>[4x]MPRIIELRQQKTAIKNQMRDMLENAEKENRSLNDAEGAKFDELRAKAESLDKDISRLEAIADEERSKPGKSSQTTDPAELRNYILTGETRALSTGVPADGGYTVIPELNTEIMRMLTDESTMRRICTVKKISSNEFKQLVSAGGATVNHGEEGKTREQTSTPQINEVSIKLYPVYAYPRTTQE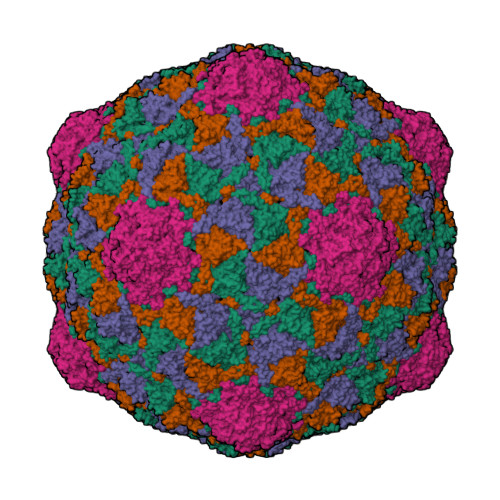IVDFSDVDILSWLTGEIGDTFTETEESDLVVGDGDKKAKGFLSVPRAEKNDKERDFGTLQVIKPSESLAWTSADPLIDLKFALRKKYRKNAVWVVNSTTAAKLQKVKNANGDYIWRDRLQAGDPDTLLGLPVEYLEFMPDNVIALGDFKRGYYIVDHETGVRTRPDNLTEPGFIKIFTQKYLGGGVVDSNAIKILELPQDDD>MINITSSASQEGTRLNLICTVWHKKEEAEGFVVFLCKDRSGDCSPETSLKQLRLKRDPGIDGVGEISSQLMFTISQVTPLHSGTYQCCARSQKSGIRLQGHFFS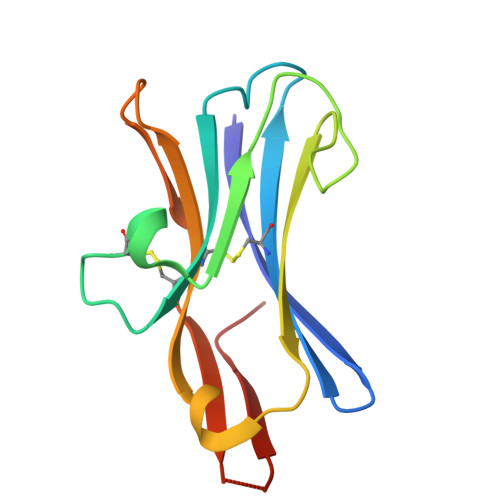ILFTETGNYTVTGLK[2x]> MTTEQRRSLQAFQDYIRKTLDPTYILSYMAPWFREEEVQYIQAEKNNKGPMEAATLFLKFLLELQEEGWFRGFLDALDHAGYSGLYEAIESWDFKKIEKLEEYRLLLKRLQPEFKTRIIPTDIISDLSECLINQECEEILQICSTKGMMAGAEKLVECLLRSDKENWPKTLKLALEKERNKFSELWIVEKGIKDVETEDLEDKMETSDIQIFYQEDPECQNLSENSCPPSEVSDTNLYSPFKPRNYQLELALPAMKGKNTIICAPTGCGKTFVSLLICEHHLKKFPQGQKGKVVFFANQIPVYEQQKSVFSKYFERHGYRVTGISGATAENVPVEQIVENNDIIILTPQILVNNLKKGTIPSLSIFTLMIFDECHNTSKQHPYNMIMFNYLDQKLGGSSGPLPQVIGLTASVGVGDAKNTDEALDYICKLCASLDASVIATVKHNLEELEQVVYKPQKFFRKVESRISDKFKYIIAQLMRDTESLAKRICKDLENLSQIQNREFGTQKYEQWIVTVQKACMVFQMPDKDEESRICKALFLYTSHLRKYNDALIISEHARMKDALDYLKDFFSNVRAAGFDEIEQDLTQRFEEKLQELESVSRDPSNENPKLEDLCFILQEEYHLNPETITILFVKTRALVDALKNWIEGNPKLSFLKPGILTGRGKTNQNTGMTLPAQKCILDAFKASGDHNILIATSVADEGIDIAQCNLVILYEYVGNVIKMIQTRGRGRARGSKCFLLTSNAGVIEKEQINMYKEKMMNDSILRLQTWDEAVFREKILHIQTHEKFIRDSQEKPKPVPDKENKKLLCRKCKALACYTADVRVIEECHYTVLGDAFKECFVSRPHPKPKQFSSFEKRAKIFCARQNCSHDWGIHVKYKTFEIPVIKIESFVVEDIATGVQTLYSKWKDFHFEKIPFDPAEMSK

RIG-I is an essential innate immune receptor for detecting and responding to infection by RNA viruses. RIG-I displays exquisite sensitivity in recognizing minute quantities of viral RNA in the cytoplasm and then forming a tight RNA:protein complex that releases specialized signaling domains (CARDs, or Caspase Recruitment Domains), which engage in a cascade of downstream interactions leading to induction of interferons and a rapid antiviral immune response. As observed in previous crystallographic studies, all complexes visualized by cryo-EM reveal a familiar ring-like structure in which the domains of RIG-I are wrapped around dsRNA and the blunt duplex terminus is capped by stacking and hydrogen-bonding networks with the protein. RIG-I selectively differentiates viral RNAs from host RNAs by adopting two different conformations, each of which is specific for a different type of RNA (host or viral).

Given that SLR30 duplexes contain a substantial “runway” for the movement of RIG-I away from the blunt duplex terminus, we wondered whether RIG-I might have a greater propensity to migrate into the center of the duplex when it starts out in the HF conformation, complexed with “host-like” RNA duplexes, such as those that terminate in a 5’-OH rather than a 5’-triphosphate. To address this question, we created a new RNA called OHSLR30, which contains a “host-like” terminus adjacent to a long duplex, and we solved a series of structures with RIG-I in the absence and presence of ATP. However, when purified OHSLR30:RIG-I complexes are incubated with ATP and Mg2+ before cryo-grid preparation, we observe two populations of molecules: A minority population (24%) that remains bound at the duplex terminus, while a majority population (76%) moves to the center of the duplex, supporting the notion that the HF conformer is a dynamically active state that readily binds ATP and assists in proof-reading. Consistent with this, the end-bound HF species contains clear density for ADP within the active-site. At the same time, with Heltnt engaged in the CTD or along the dsRNA backbone, the Hel2 domain remains well-folded in these complexes, enabling them to engage with ATP and stimulating active RNA dissociation or translocation away from the high-affinity terminus. Rapid off-rate from these host sites is further enhanced by active cycles of ATP binding and hydrolysis that further accelerate RNA dissociation and, in some cases, cause RIG-I to move away from the terminus to even lower affinity sites on the duplex interior.>SNATLREQSFDEAWLFHRGDIAEGEKQSLDDSQWRQINLPHDWSIEDIPGTNSPFTADAATEVAGGFTVGGTGWYRKHFYIDAA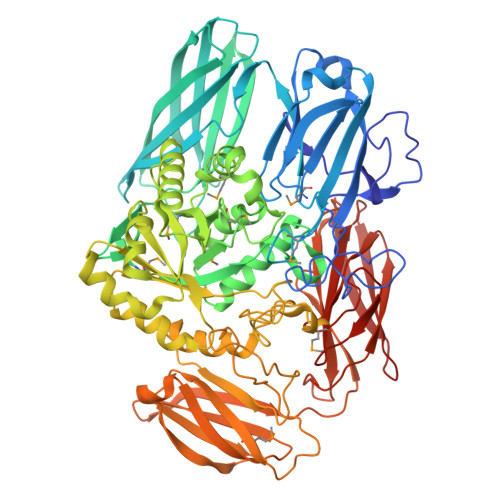EKGKCIAVSFDGIYMNADIWVNDRHVANHVYGYTAFELDITDYVRFGAENLIAVRVKNEGMNCRWYTGSGIYRHTFLKITNPLHFETWGTFVTTPVATADKAEVHVQSVLANTEKVTGKVILETRIVDKNNHTVARKEQLVTLDNKEKTEVGHALEVLAPQLWSIDNPYLYQVVNRLLQDDKVIDEEYISIGIRNIAFSAENGFQLNGKSMKLKGGCIHHDNGLLGAKAFDRAEERKIELLKAAGFNALRLSHNPPSIALLNACDRLGMLVIDEAFDMWRYGHYQYDYAQYFDKLWKEDLHSMVARDRNHPSVIMWSIGNEIKNKETAEIVDICRELTGFVKTLDTTRPVTAGVNSIVDATDDFLAPLDVCGYNYCLNRYESDAKRHPDRIIYASESYASQAYDYWKGVEDHSWVIGDFIWTAFDYIGEASIGWCGYPLDKRIFPWNHANCGDLNLSGERRPQSYLRETLWSDAPVSHIVVTPPVPSFPLNPDKADWSVWDFPDVVDHWNFPGYEGKKMTVSVYSNCEQVELFLNGESLGKQENTADKKNTLVWEVPYAHGILKAVSYNKGGEVGTATLESAGKVEKIRLSADRTEIVADGNDLSYITLELVDSKGIRNQLAEELVAFSIEGDATIEGVGNANPMSIESFVANSRKTWRGSNLLVVRSGKSSGRIIVTAKVKALPVASITITQKK[2x]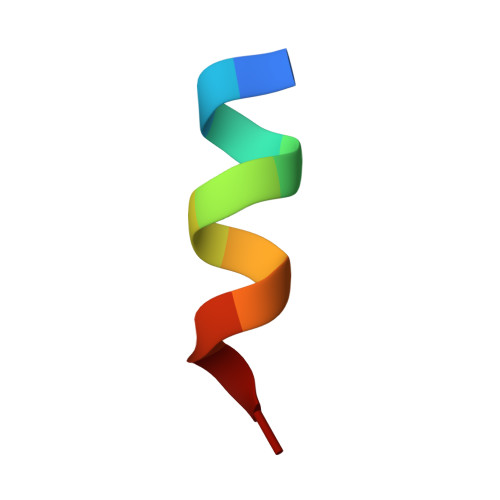> DAIDALSSDFT> AAPDSQVCDVGSTATCKITATPRQFQPALLSTSKWIWTGENPIPGGSNIISTRPFRKNITAPCGKCSVCATIVVASDDAHTFYVNGVRIGTGAGFRQGQALFVALQPTWNLFAIAGQNLVANSPAGIMASILVHFSDGTSETFVTDESWKTLRAAPPENFQLPSTNDSNWPSAAVQGAYQNSVWGPPVLPPVLPLRGSNWIWTSDNVNGAAPVGSRAFRKTV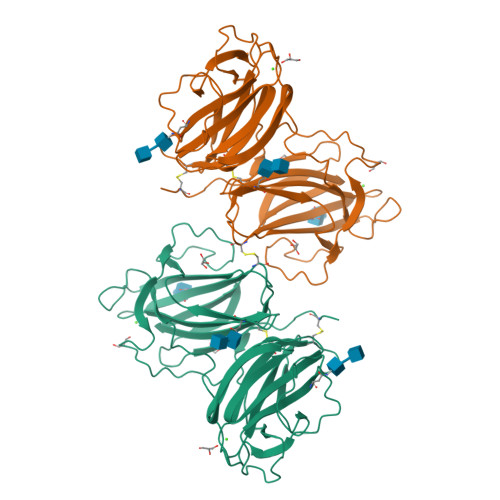NQCTKVAVCATVLIAADDRYTLYVNGATVGSGSSYTVADAYTIPNLHPTFNTFAINATNGGGPAGVIATILITYSDGSNETVVTDASWKAIQTIPQGFQPPLIDEFGWESAKIIGAFGVAPWGAGMVIPSA>RMEIVKIPVVVHVVWNEEEENISDAQIQSQIDILNKDFRKLNSDVSQVPSVWSNLIADLGIEFFLATKDPNGNQTTGITRTQTSVTFFTTSDEVKFASSGGEDAWPADRYLNIWVCHVLKSEIGQDILGYAQFPGGPAETDGVVIVDAAFGTTGTALPPFDKGRTATHEIGHWLNLYHIWGDELRFEDPCSRSDEVDDTPNQADPNFGCPSYPHVSCSNGPNGDMFMNYCDYVDDKCMVMFTQGQATRVNACLDGPRSSFLA[2x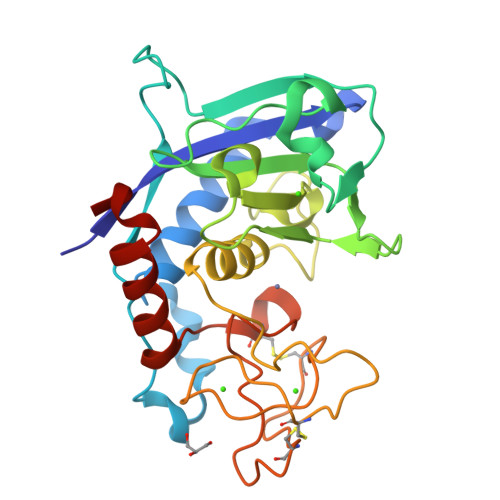]> MSQVKIYANERTIIQYRELLSHAIHQALIEELKYPVEKRFQRFISLKPENFIYPSDRSQHYIIIELSMFAGRSPATKKQLIQTLFRNIEEQC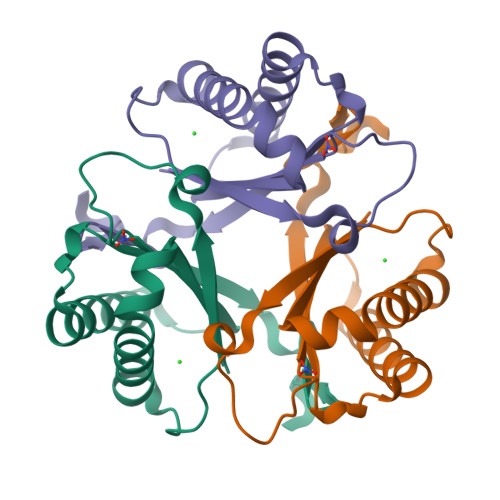KIAPQDIEITIFETPKENWGIRGKNADELLLNYQVNI>MSQSNRELVVDFLSYKLSQKGYSASGGGGGGGMAAVKQALREAGDEFELRYRRAFSDLTSQLHITPGTAYQSFEQVVNELFRDGVNWGRIVAFFSFGGALCVESVDKKMQVLVSRIAAWMATYLNDHLEPWIQENGGWATFVELYGNNA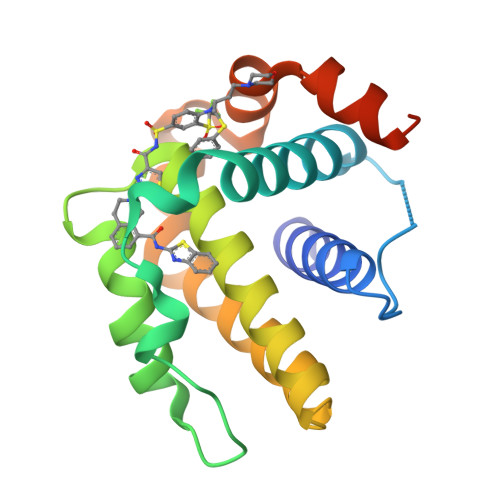AAESRKGQERLEHHHHHH[2x]>MLY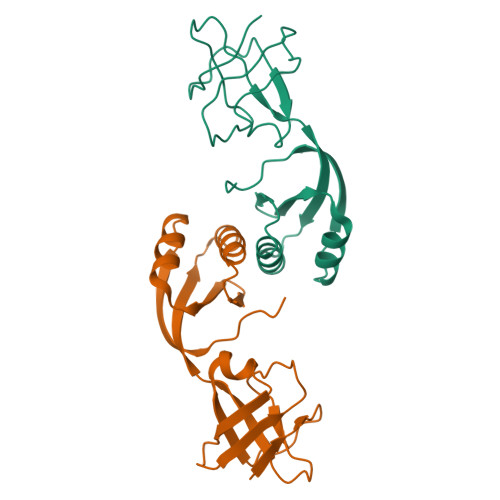LTQRLEIPAAATASVTLPIDVRVKSRVKVTLNDGRDAGLLLPRGLLLRGGDVLSNEEGTEFVQVIAADEEVSVVRCDDPFMLAKACYHLGNRHVPLQIMPGELRYHADHVLDDMLRQFGLTVTFGQLPFEPEAGAYASES[2x]>[6x]MNYLNNIRIENPLTICYTNDVVKNFTANGLLSIGASPAMSEAPEEAEEFYKVAQALLINIGTLTAQNEQDIIAIAQTANEAGLPIVFDPV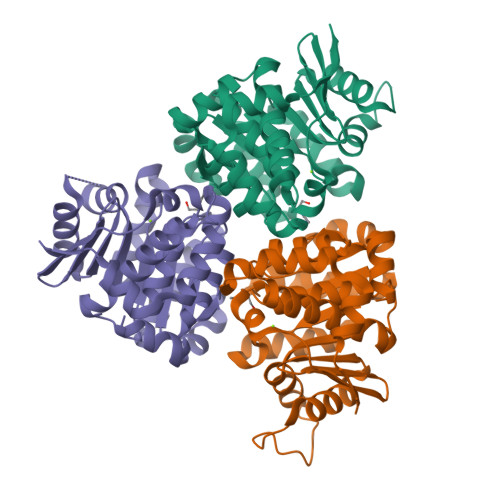AVGASTYRKQFCKLLLKSAKVSVIKGNASEILALIDDTATMKGTDSDANLDAVTIAKKAYAIYKTAIVITGKEDVIVQGDKAIVLANGSPLLARVTGAGCLLGGIIAGFLFRETEPDIEALIEAVSVFNIAAEVAAENENCGGPGTFSPLLLDTLYHLNETTYQQRIRIQEVEENLYFQSGHHHHHH> GEFETLEQLKESLKKE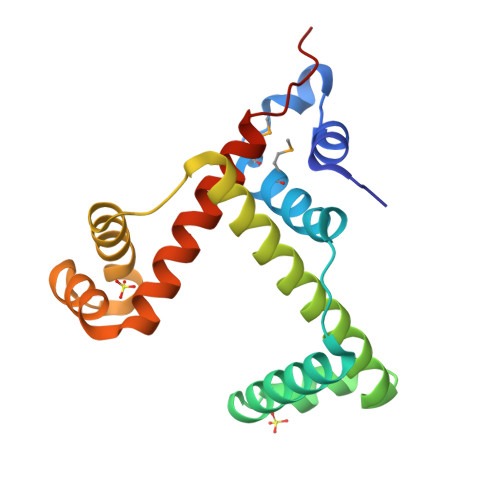GKEIYDVEMKESMREQLLEKLPEIVEIEISDRTLEILVNEAINRLKREGRYEQIVSSYESEEKFREELKERILDDIKRDRVIEVLAQEKGISVNDEELEKEAEELAPFWGISPDRAKSLVKARQDLREELRWAILKRKVLDLLLQEVEHHHHHH>[2x]MSLIASIGELLIDLI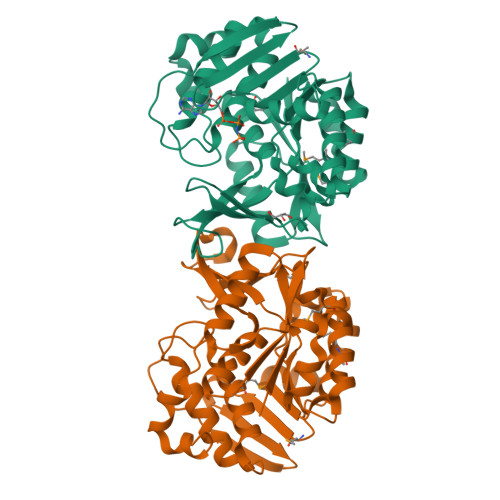SVEEGDLKDVRLFEKHPGGAPANVAVGVSRLGVKSSLISKVGNDPFGEYLIEELSKENVDTRGIVKDEKKHTGIVFVQLKGASPSFLLYDDVAYFNMTLNDINWDIVEEAKIVNFGSVILARNPSRETVMKVIKKIKGSSLIAFDVNLRLDLWRGQEEEMIKVLEESIKLADIVKASEEEVLYLENQGVEVKGSMLTAITLGPKGFRLIKNETVVDVPSYNVNPLDTTGAGDAFMAALLVGILKLKGLDLLKLGKFANLVAALSTQKRGAWSTPRKDELLKYKEAREVLAEGHHHHHH>MKNWQRIVEAKLEQQKHKVAEISLENGTVNYSKKIKHNRNLKALTGDEEIVRAFLIDRLVNELDYKPEYLETEKEYTIKGGHSKINPRVDVLVKDDKGNPFFFIEVKAPNKFEEDKDEIEGQLFALAQAEERDFKTKVKYLVYYTVELIDDEIVDRAIIIDFEKYPTYTDWSNGGFISTGTELTAGYGEPKKQPLIKGHEKYDLRVRIDREEIEGLGRNLHNVLWGGGGTNDSEIFYSLVNIILAKIQDEYEKEDGQEYDFQVYQYGDNVESPQKLFDRINALYKRALREQLNVTDEQKIAEDNVINRNKFPLNKLVYTVQALESLSFLEGRNSLDGKDILGDFFESIIRDGFKQTKGQFFTPTPIVKFILYALQLDKLAIDRLNNDRELPLIIDPSAGSGTFLIEAMKLITKEVKYKQNHKVKSSRQITKRFEELFMPDHNENKWAREYLYGCEINFDLGTASKVNMILHGDGSANIFVQDGLLPFRFYVKETSPNYLETASPDALYGDKEVNGKFDVVVSNPPFSVDLDTQTQREVRNAFLFGDKKNSENLFIERYYQLLKEGGRLGVVLPESVFDTTENKYIRLF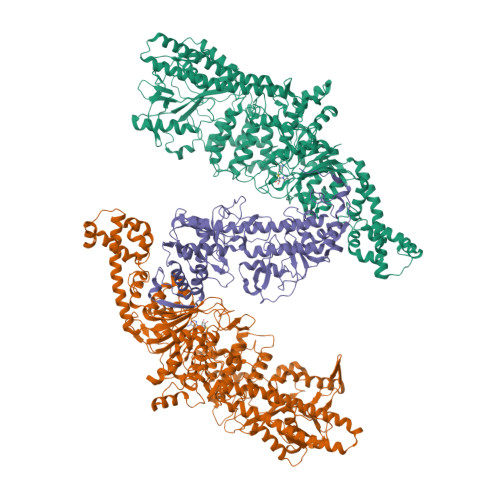IFKYFKVKAVVSLPQVTFEPFTSTKTSLLFAQKKTKEEVEQWNELWDKYGKEWSLLKTRINDYFSYFVKGRPLNKKWAPDVVKDIQEGNEDNIRKNIFRFLKDHIKEEDKNLEIKDLLIKYAEEISSISKHEKETDVFGFYNAWWVFGEVAKELDYPIFMAEAENVGYKRTKKGEKPMPNDLYDLEYAPSTLDCEKVLSSFDIEINALEASKTKLSVEKGLLEEKLKDKEDKENEKIQKRLNKISELLETIENQLDSIRSKKLEVEGILEKYYENNKLKEEYSERDDEELINHFKHGVLYQYRSEDILLRNKTVHKILDEIRQGVIWD[2x];> MGLIQRRNFSTFASEPSVRFDFNYMKSVTPTTEEYYTYKSLFEVVPSTVPTLDESEPFKYAEIGHVSKNGEVFPVTLSFEDRDELNEDLFKKIEKGDIFLPERGNILISAIRPYLNKIVLIKEDDKTDIYFTKAFIQIKPLINSRILYYALRTIFSEKINAVSRQGKGYPTLKEDDLKTIQFSKKVIDNLLAKEEELISNIDALEKDIKELKSIQRSKKEIVDEVFSSHFNINMVELMALDSQRRVDVGLSSISSLNSTIRYSYRWNKMKLIQKYLYRDIDCIEPLGKYILSSNNGWSPESVVGGEGIPILGQEHLEFDGVLNVSPTKATTKTKNNMENFFIQEGDLFISRGNTVDLVGLACVVETEVTEDIIYPDLYIRLKIDEKVIHKKYLALLFNSFFGRLYFKYVSKGKNQTMVKISSNELLNYYLPIPPMEEQLEIVGKIEEQIGAQNEIEKQIEEKRNQIRVIIEETARS> MDVVSLDKPFMYFEEIDNELDYEPESANEVAKKLPYQGQLKLLLGELFFLSKLQRHGILDGATVVYIGSAPGTHIRYLRDHFYNLGVIIKWMLIDGRHHDPI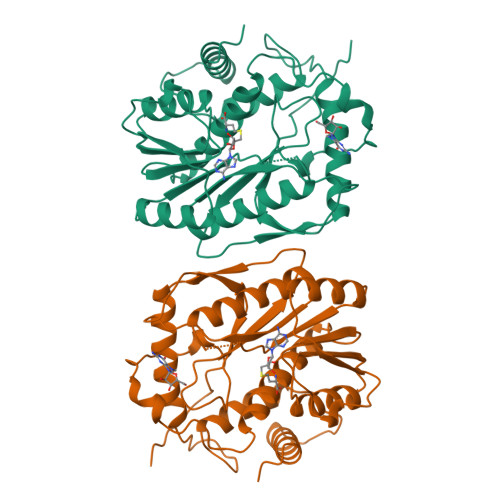LNGLRDVTLVTRFVDEEYLRSIKKQLHPSKIILISDVRSKRGGNEPSTADLLSNYALQNVMISILNPVASSLKWRCPFPDQWIKDFYIPHGNKMLQPFAPSYSAEMRLLSIYTGENMRLTRVTKSDAVNYQKKMYYLNKIVRNKVVVNFDYPNQEYDYFHMYFMLRTVYCNKTFPTTKAKVLFLQQSIFRFLNIP> DPFTQFKQTPLPYAYDALEGAIDAKTMEIHYSKHHAGYTANLNKAIAGTPAEKESIENILAKVSQYSDAVRNNAGGHYNHELFWSILTPNKGTKPSAALQKAIDETFGSLDALKEKINAAGAARFGSGWAWLIVDNGGKLQVTSTPNQDNPLMDFTKEKGTPILGIDVWEHAYYLRYQNKRADYLTTIWDVINWEEVSARYEKAL;> DPFTQFKQTPLPYAYDALEGAIDAKTMEIHYSKHHAGYTANLNKAIAGTPAEKESIENILAKVSQYS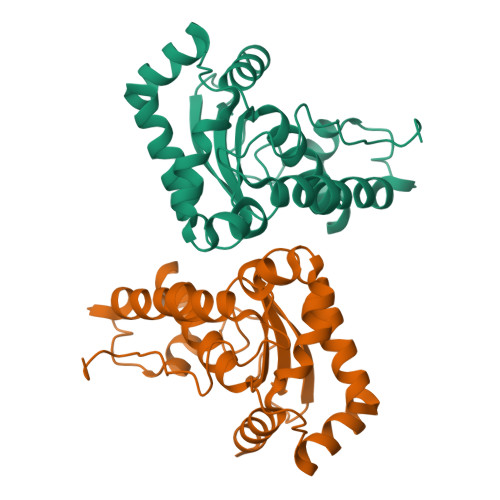DAVRNNAGGHYNHELFWSILTPNKGTKPSAALQKAIDETFGSLDALKEKINAAGAARFGSGWAWLIVDNGGKLQVTSTPNQDNPLMDFTKEKGTPILGIDVWEHAYYLRYQNKRADYLTTIWDVINWEEVSARYEKALK> MGSDKIHHHHHHNTPREVTLHFLRTAGHPLTRWALQRQPPSPKQLEEEFLKIPSNFVSPEDLDIPGHASKDRYKDILPNPQSRVCLGRAQSQEDGDYIN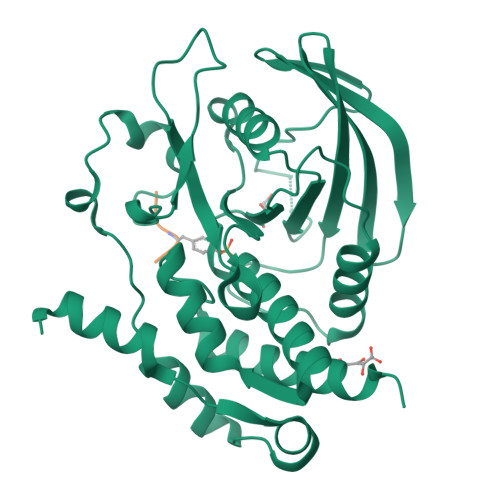ANYIRGYDGKEKVYIATQGPMPNTVSDFWEMVWQEEVSLIVMLTQLREGKEKCVHYWPTEEETYGPFQIRIQDMKECPEYTVRQLTIQYQEERRSVKHILFSAWPDHQTPESAGPLLRLVAEVEESPETAAHPGPIVVHSSAGIGRTGCFIATRIGCQQLKARGEVDILGIVCQLRLDRGGMIQTAEQYQFLHHTLALYAGQLPEEPSP;> LTEYVATR>GAMGSMAEAEGESLESWLNKATNPSNRQEDWEYIIGFCDQINKELEGPQIAVRLLAHKIQSPQEWEALQALTVLEACMKNCGRRFHNEVGKFRFLNELIKVVSPKYLGDRVSEKVKTKVIELLYSWTMALPEEAKIKDAYHMLKRQ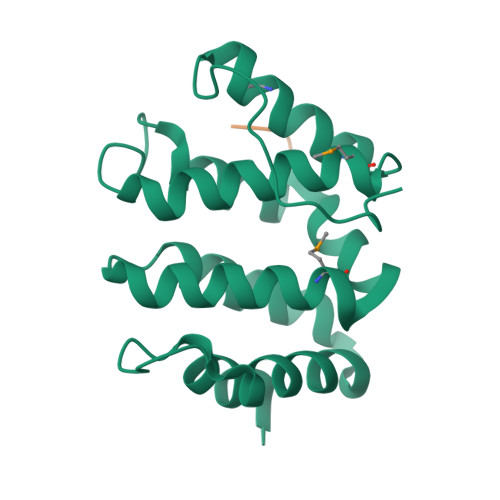GIVQSDPPIPVDRTLIPSPPPRPKN[4x];>EESEERDDHLLPM[4x]>[4x]GPRTRIPYKPNYSLNLWSIMKNCIGKELSKIPMPVNFNEPLSMLQRLTEDLEYHELLDRAAKCENSLEQLCYVAAFTVSSYSTTVFRTSKPFNPLLGETFELDRLEENGYRSLCEQVSHHPPAAAHHAESKNGWTLRQEIKITSKFRGKYLSIMPLGTIHCIFHATGHHYTWKKVTTTVHNIIVGKLWIDQSGEIDIVNHKTGDKCNLKFVPYSYFSRDVARKVTGEVTDPS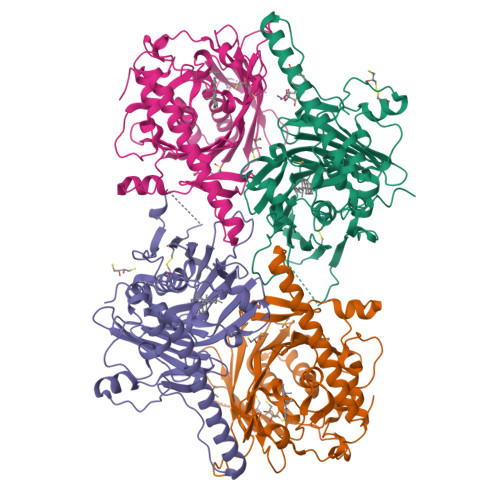GKVHFALLGTWDEKMECFKVQPVIGENGGDARQRGHEAEESRVMLWKRNPLPKNAENMYYFSELALTLNAWESGTAPTDSRLRPDQRLMENGRWDEANAEKQRLEEKQRLSRKKREAEAMKATEDGTPYDPYKALWFERKKDPVTKELTHIYRGEYWECKEKQDWSSCPDIF>SNAMIIRPEQHWFLRLFDWHGSVLSKIIFRLLLNVLMSIIAIISYQWYEQLGIHLTVAPFSLLGIAIAIFLGFRNSASYSRFVEARNLWGTVLIAERTLVRQLRNILPAEHDAHRRIVSYLVAFSWSLKHQLRKTDPTADLRRLLPEERVTEILASSMPTNRILLLAGNEIGQLREAGKLSDITYGLMDNKLDELAHVLGGCERLATTPVPFAYTLILQRTVYLFCTLLPFALVGDLHYMTPFVSVFISYTFLSWDSLAEEAEDPFGTAANDLPLNAMCNTIERNLLDMTGQHPLPE[5x]

Human bestrophin1 (hBest1) is a Ca2+-activated Cl− channel essential for Cl− transport in retinal pigment epithelium (RPE). Although the structure of hBest1 is still unsolved, two Best1 homolog structures, one from bacteria Klebsiella pneumoniae (KpBest) and the other from chicken (cBest1), have been previously reported. Overall, the channel is a pentameric assembly with a single ion-conducting pathway, which varies in diameter along its length and is constrained at two narrow points: a “neck” contributed by three residues (I62/I66/F70 in KpBest and I76/F80/F84 in hBest1/cBest1) on a transmembrane helix, and an “aperture” formed by a single residue (I180 in KpBest1, I205 in hBest1, and V205 in cBest1) on a cytosolic helix. Here, by electrophysiological and structural analyses, we show that the neck and aperture in hBest1 are both indispensable Ca2+-dependent gates, and their dysregulated opening by rationally designed or patient-derived mutations causes Ca2+-independent leak and elevates Ca2+-dependent channel activity.

Alanine substitution mutants for each of the 12 residues were generated in KpBest and hBest1 and subjected to crystallography and patch clamp, respectively. Moreover, the equivalent KpBest mutants (W16A, G18A, S19A, L259A, P262A, G264A, and D269A) all showed an overall similar structure to that of WT KpBest. The corresponding “Ca2+-binding” sites in WT KpBest are occupied by Zn2+, an essential component in the crystallization buffer. Moreover, KpBest L259A, P262A, G264A, and D269A all have relatively low resolution and slightly altered structures in this region, suggesting that the binding of Zn2+ stabilizes the channel structure.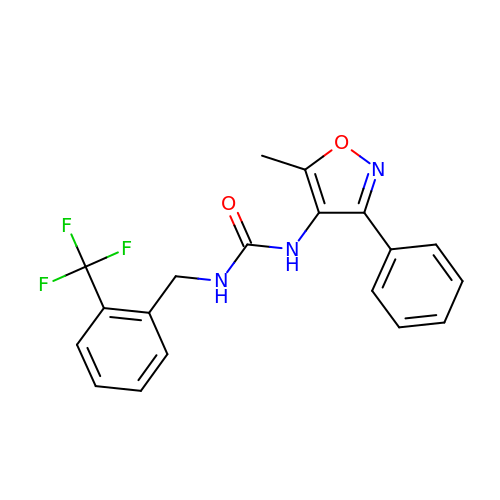1-(5-methyl-3-phenyl-1,2-oxazol-4-yl)-3-[[2-(trifluoromethyl)phenyl]methyl]urea | C19 H16 F3 N3 O2 | JOPADRLBMVFGBD-UHFFFAOYSA-N> MAQRKNAKSSGNSSSSGSGSGSTSAGSSSPGARRETKHGGHKNGRKGGLSGTSFFTWFMVIALLGVWTSVAVVWFDLVDYEEVLGKLGIYDADGDGDFDVDDAKVLLGLKERSTSEPAVPPEEAEPHTEPEEQVPVEAEPQNIEDEAKEQIQSL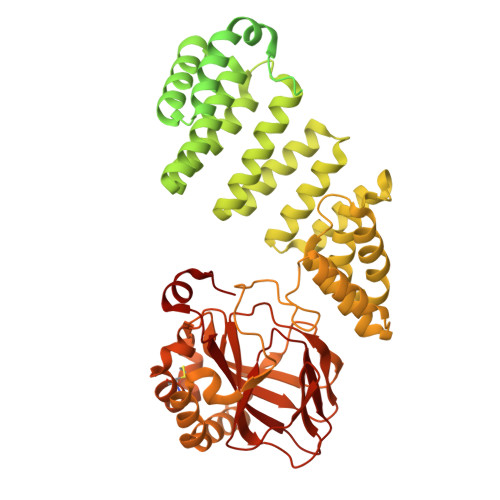LHEMVHAEHVEGEDLQQEDGPTGEPQQEDDEFLMATDVDDRFETLEPEVSHEETEHSYHVEETVSQDCNQDMEEMMSEQENPDSSEPVVEDERLHHDTDDVTYQVYEEQAVYEPLENEGIEITEVTAPPEDNPVEDSQVIVEEVSIFPVEEQQEVPPETNRKTDDPEQKAKVKKKKPKLLNKFDKTIKAELDAAEKLRKRGKIEEAVNAFKELVRKYPQSPRARYGKAQCEDDLAEKRRSNEVLRGAIETYQEVASLPDVPADLLKLSLKRRSDRQQFLGHMRGSLLTLQRLVQLFPNDTSLKNDLGVGYLLIGDNDNAKKVYEEVLSVTPNDGFAKVHYGFILKAQNKIAESIPYLKEGIESGDPGTDDGRFYFHLGDAMQRVGNKEAYKWYELGHKRGHFASVWQRSLYNVNGLKAQPWWTPKETGYTELVKSLERNWKLIRDEGLAVMDKAKGLFLPEDENLREKGDWSQFTLWQQGRRNENACKGAPKTCTLLEKFPETTGCRRGQIKYSIMHPGTHVWPHTGPTNCRLRMHLGLVIPKEGCKIRCANETKTWEEGKVLIFDDSFEHEVWQDASSFRLIFIVDVWHPELTPQQRRSLPAI> RPESELIRQSWRVVSRSPLEHGTVLFARLFALEPSLLPLFQYNGRQFSSPEDSLSSPEFLDHIRKVMLVIDAAV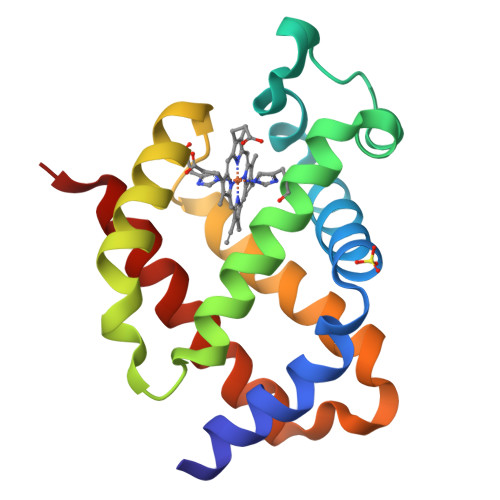TNVEDLSSLEEYLTSLGRKHRAVGVRLSSWSTVGESLLYMLEKSLGPDFTPATRTAWSRLYGAVVQAMSRGWDGE> MNPIHDRTSDYHKYLKVKQGDSDLFKLTVSDKRYIWYNPDPKERDSYECGEIVSETSDSFTFKTVDGQDRQVKKDDANQRNPIKFDGVEDMSELSYLNEPAVFHNLRVRYNQDLIYTYSGLFLVAVNPFKRIPIYTQEMVDIFKGRRRNEVAPHIFAISDVAYRSMLDDRQNQSLLITGESGAGKTENTKKVIQYLASVAGRNQANGSGVLEQQILQANPILEAFGNAKTTRNNNSSEFGKFIEIQFNSAGFISGASIQSYLLEKSRVVFQSETERNYHIFYQLLAGATAEEKKALHLAGPESFNYLNQSGCVDIKGVSDSEEFKITRQAMDIVGFSQEEQMSIFKIIAGILHLGNIKFEKGAGEGAVLKDKTALNAASTVFGVNPSVLEKALMEPRILAGRDLVAQHLNVEKSSSSRDALVKALYGRLFLWLVKKINNVLCQERKAYFIGVLDISGFRIFKVNSFEQLCINYTNEKLQQFFNHHMFKLEQEEYLKEKINWTFIDFGLDSQATIDLID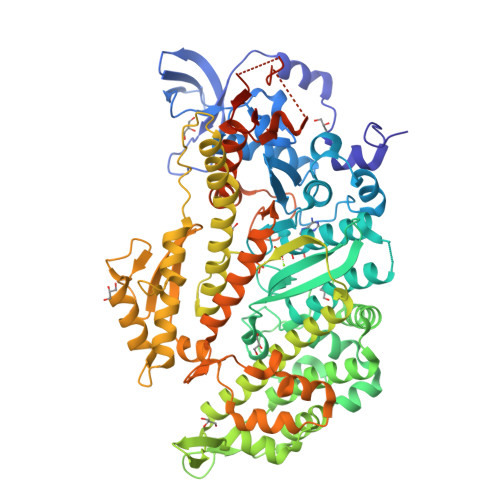GRQPPGILALLDEQSVFPNATDNTLITKLHSHFSKKNAKYEEPRFSKTEFGVTHYAGQVMYEIQDWLEKNKDPLQQDLELCFKDSSDNVVTKLFNDPNIASRAKKGANFITVAAQYKEQLASLMATLETTNPHFVRCIIPNNKQLPAKLEDKVVLDQLRCNGVLEGIRITRKGFPNRIIYADFVKRYYLLAPNVPRDAEDSQKATDAVLKHLNIDPEQYRFGITKIFFRAGQLARIEEAREQRDYKDDDDK>[2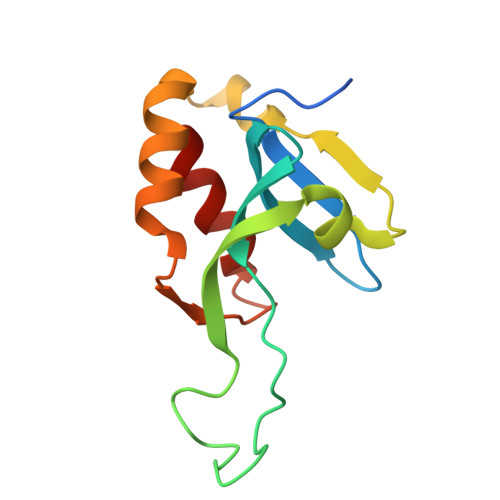x]GPGMASPHQEPKPGDLIEIFRLGYEHWALYIGDGYVIHLAPPSEYPGAGSSSVFSVLSNSAEVKRERLEDVVGGCCYRVNNSLDHEYQPRPVEVIISSAKEMVGQKMKYSIVSRNCEHFVTQLRYG>[10x]METVVGLTAIAVALLIGLGALGTAIGFGLLGGKFLEGAARQPEMVPMLQVKMFIVAGLLDAVTMIGVGIALFFTFANPFVGQIAG;>MNINATLIGQSVAFFIFVLFCMKFVWPPVIAALQERQKKIADGLDAANRAARDLELAHEKAGQQLREAKAQAAEIVEQAKKRANQIVDEARDQARTEGERLKAQAQAEIEQELNSV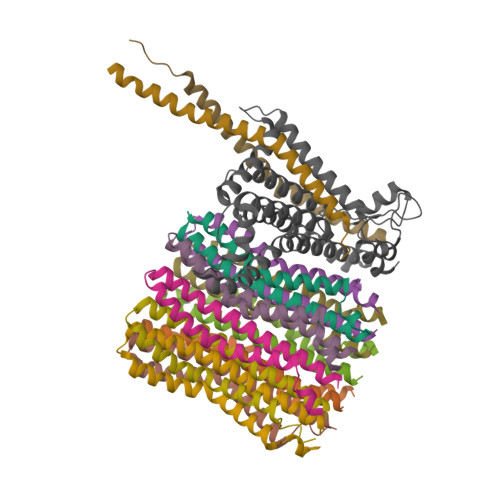KDALRAQVGALAVTGAEKILGASIDANAHEQLVSKLAAEI[2x];> MAAETASGYIQHHLQNLTFGRLPNGDWGFAHTAEQAKEMGFWAFHVDTLGWSVLLGVVFLFIFRLAAKKATSGQPGGLQNFVEVMVEFVDTSVKDTFHGRNPLIAPLALTVFVWIFLLNLIDLVPVDYLPMLAAKITGDEHLFFRAVATTDPNATLGLSISVFALIVFYSIKVKGIGGFLGELTLHPFSSKNIVVQILLIPVNFLLEFVTLIAKPVSLALRLFGNMYAGELIFILIAVMFGSGMFLLSALGVALNWAWAVFHILIITLQAFIFMMLTIVYLSMAHEDNH>ELCNPQDKQALLQIKKDLGNPTTLSSWLPTTDCCNRTWLGVLCDTDTQTYRVNNLDLSGLNLPKPYPIPSSLANLPYLNFLYIGGINNLVGPIPPAIAKLTQLHYLYITHTNVSGAIPDFLSQIKTLVTLDFSYNALSGTLPPSISSLPNLVGITFDGNRISGAIPDSYGSFSKLFTSMTISRNRLTGKIPPTFANLNLAFVDLSRNMLEGDASVLFGSDKNTQKIHLAKNSLAFDLGKVGLSKNLNGLDLRNNRIYGTLPQGLTQLKFLHSLDVSFNNLCGEIPQGGNLQRFDVSAYANNKCLCGSPLPACT[4x];>[4x]DPCSVTEYSGLATAVSSCKNIVLNGFQVPTGKQLDLSSLQNDSTVTFKGTTTFATTADNDFNPIVISGSNITITGASGHVIDGNGQAYWDGKGSNSNSNQKPDHFIVVQKTTGNSKITNLNIQNWPVHCFDITGSSQLTISGLILDNRAGDKPNAKSGSLPAAHNTDGFDISSSDHVTLDNNHVYNQDDCV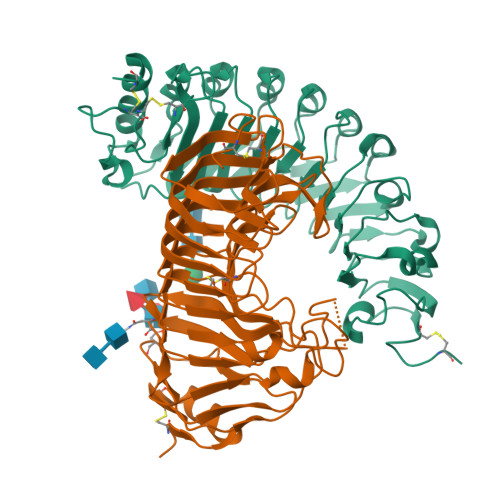AVTSGTNIVVSNMYCSGGHGLSIGSVGGKSDNVVDGVQFLSSQVVNSQNGCRIKSNSGATGTINNVTYQNIALTNISTYGVDVQQDYLNGGPTGKPTNGVKISNIKFIKVTGTVASSAQDWFILCGDGSCSGFTFSGNAITGGGKTSSCNYPTNTCPS> MSSAVEKKDLPADYGKMPAGYNFLTRGKDWREYDKDFILRTDAVWEKFQLEHFFRNYMKCFFFDHGLKKYQMFEPEDMYTVVFEGWALDDLITFPGFTPTGRT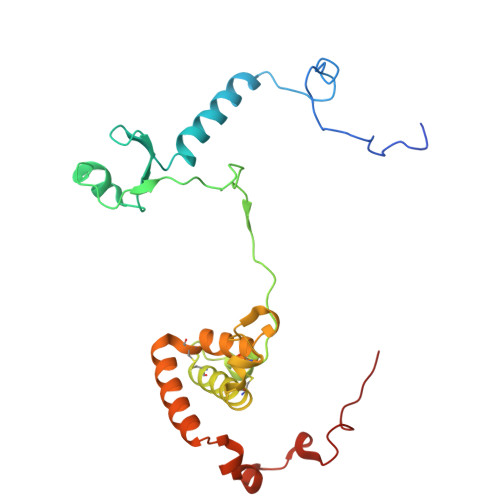NSYQIGLSPRQRTVVPTQTFYQMQDYYMLCGLRFERWFRCDLVYHDQRHTKFDQVKNQKNYKTYPCYREYYEAQYACQDDMFDFLMELAYARRAADNFESDFASHELTTLPTFYDTPKAAERKTYTY>[3x]GPGSVRVVRGRGLLRAVLDRPERRNPIDAGLLTSLARALDQAESDQDCRVFVLSSTGEDFCAGTDLSGGDPAPE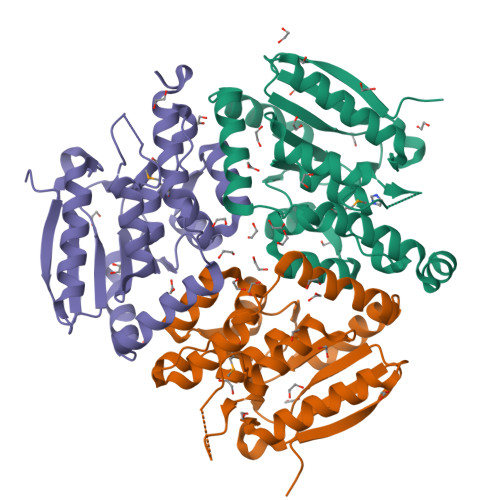PLPDGAELPYWTLLERLTRSPLATVAVVDGRATAGGVGLAAACDLVLAGERARFRLTEVLAGLVPAMALPFVARRTGEQRAFAATLRAEEFDAGAAHRVGLADLAGPRAEDLLPPVLAGLGRTDRSTTAALKEYRARLFPRDARLGHDASRLLIERFAAPGTGQLLARLREAGAAA> LPTAQEVQGLM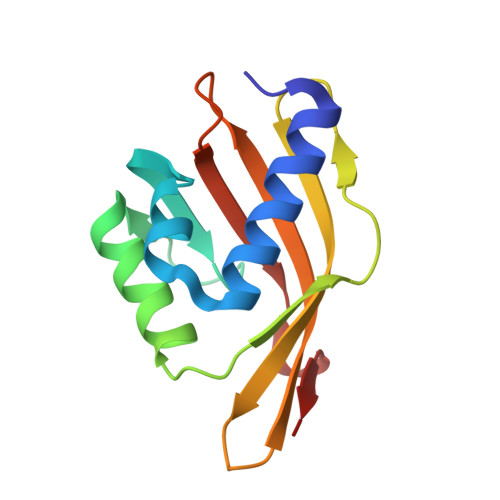ARYIELVDVGDIEAIVQMYADDATVEDPFGQPPIHGREQIAAFYRQGLGGGKVRACLTGPVRASHNGCGAMPFRIEMVWNGQPCAVDAISVMRFDEHGRIQTMQAYWSEVNLSV>[2x]GSDVVDPDIFNRDPRDHYDLLQRLGGGTYGEVFKARDKVSGDLVALKMVKMEPDDDVSTLQKEILILKTCRHANIVAYHGSYLWLQKLWICMEFCGAGSLQDIYQVTGSLSELQISYVCREVLQGLAYLHSQKKIHRDIKGANILINDAGEVRLADFGISAQIGAELARRLEFIGTPYWMAPEVAAVALKGGYNELCDIWSLGITAIELAELQPPLFDVHPLRVLFLMTKSGYQPPR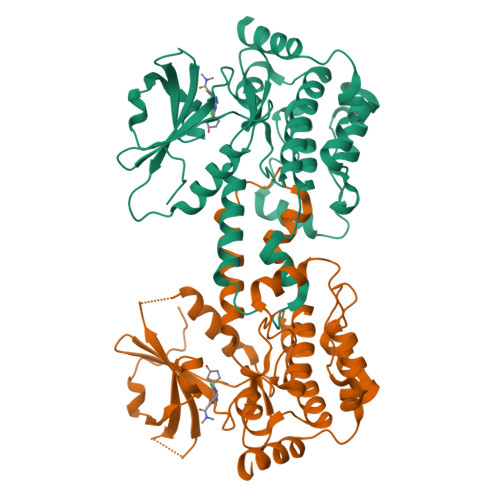LKEKGKWSAAFHNFIKVTLTKSPKKRPSATKMLSHQLVSQPGLNRGLILDLLDKLKNGNS Clostridium thermocellum has extensive potential in lignocellulose biorefineries as an environmentally prominent, thermophilic, cellulolytic bacterium. Previously, five putative sugar transporters, denoted A to D and L and belonging to the ABC transport systems group, were identified in the genome of C. thermocellum, and the solute-binding lipoproteins (SBP) of these ABC transporters were shown to bind different dextrins by isothermal titration calorimetry (ITC) assays. To gain insight into the structural mechanism of the transporter specificities, 11 crystal structures, both alone and in complex with appropriate saccharides, were solved for all 5 putative sugar-binding proteins, thus providing detailed specific interactions between the proteins and the corresponding saccharides. Combined genetic, biophysical, and structural studies have provided solid evidence that transporter A and transporter B are the major glucose and cellodextrin transporters, respectively, among the five potential sugar transporters in C. thermocellum.

The unliganded CbpC and CbpD structures were determined to 2.00 and 1.50 Å resolution, respectively. A Dali search using the CbpD structure revealed similarity with several monosaccharide-binding proteins in the closed conformation. A nearly closed substrate-binding pocket between domains I and II was found in the unliganded CbpD crystal structure, which is suitable for accommodating a monosaccharide. The small substrate-binding pocket suggests that CbpD cannot bind to cellodextrin, in agreement with our titration and genetic experimental results. CbpD has been proposed to be the transporter of xylose, but we could not detect any xylose-binding ability in either ITC or NMR experiments. For CbpC and CbpD, no interaction was detected for all of the tested carbohydrate substrates in both ITC and NMR experiments, suggesting that transporters C and D are not responsible for glucose or cellodextrin transport.

> SVLVGCGNNTTNNNSGTSGPSTNSGTSGSGTNSGTTSNNVTGKTDLADTNFDTSYTPKRTSYKIYCTYKNIHAWYDAIKCGIDAAVKELAEKGVTVDYEWYGPAQPDAVDQVNSIETAIGQGWDLIAVDVNQPELTGEAINNAVAKGIPVAVFGTSDVPNCDRAFFVGNTDPYGDGCALAKAVCEKMGGKGQIAILAGTIGALAHEERLRGFKDTIAKYPDIEIVDEQRDNDEVEKAISITESWLQAYPNLGGILCNNMSNPVGACQAVADAGKSGKIVIGGMDHDLRALNALKDGTLYVAQVQNCYDMGYKLIYNAIKTIDGEKVEESTAVGSTSVYAQDADKFINMLYGEAN> KLPPGPTPLPVIGNILQIGIKDISKSLTNLSKVYGPVFTLYFGLKPIVVLHGYEAVKEALIDLGEEFSGRGIFPLAERANRGFGIVFSNGKKWKEIRRFSLMTLRNFGMGKRSIEDRVQEEARCLVEELRKTKASPCDPTFILGCAPCNVICSIIFHKRFDYKDQQFLNLMEKLNENIKILSSPWIQICNNFSPIIDYFPGTHNKLLKNVAFMKSYILEKVKEHQESMDMNNPQDFIDCFLMKMEKEKHNQPSEFTIESLENTAVDLFGAGTETTSTTLRYALLLLLKHPEVTAKVQEEIERVIGRNRSPCMQDRSHMPYTDAVVHEVQRYIDLLPTSLPHAVTCDIKFRNYLIPKGTTILISLTSVLHDNKEFPNPEMFDPHH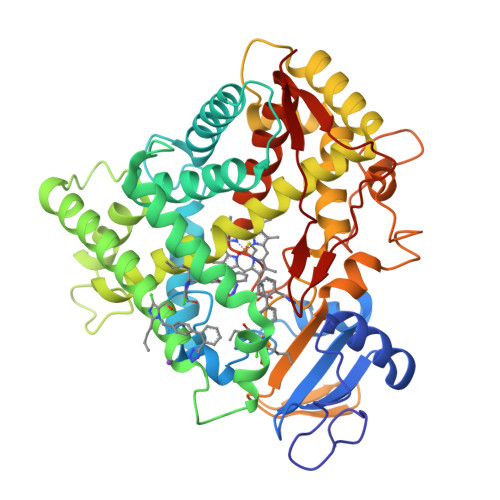FLDEGGNFKKSKYFMPFSAGKRICVGEALAGMELFLFLTSILQNFNLKSLVDPKNLDTTPVVNGFASVPPFYQLCFIPI>MKFGLFFLNFMNS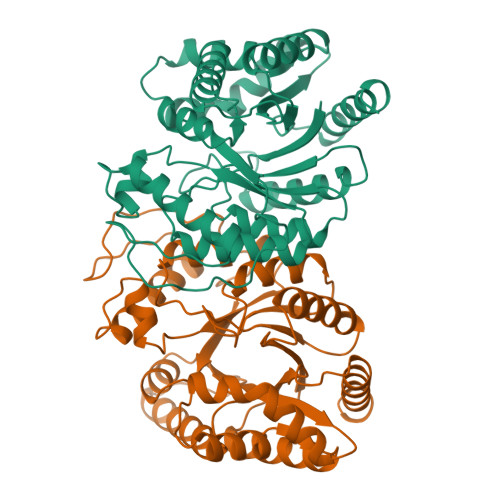KRSSDQVIEEMLDTAHYVDQLKFDTLAVYENHFSNNGVVGAPLTVAGFLLGMTKNAKVASLNHVITTHHPVRVAEEACLLDQMSEGRFAFGFSDCEKSADMRFFNRPTDSQFQLFSECHKIINDAFTTGYCHPNNDFYSFPKISVNPHAFTEGGPAQFVNATSKEVVEWAAKLGLPLVFRWDDSNAQRKEYAGLYHEVAQAHGVDVSQVRHKLTLLVNQNVDGEAARAEARVYLEEFVRESYSNTDFEQKMGELLSENAIGTYEESTQAARVAIECCGAADLLMSFESMEDKAQQRAVIDVVNANIVKYHS[2x]In response to environmental stimuli, the bacterium produces and secretes its main virulence factor, the cholera toxin (CT). CT is an AB5 protein toxin, which consists of one toxic A-subunit (CTA) and five identical B-subunits arranged in a doughnut-shaped ring (CTB). The primary receptor of the cholera toxin is the GM1 ganglioside, which is expressed in distinct membrane microdomains of small-intestinal epithelial cells. There are two major biotypes of V. cholerae, classical and El Tor, which produce cholera toxins with a slight sequence variation (cCT and ET CT). cCT and ET CT differ in only two residues of the B-subunit, His18/Tyr18 and Thr47/Ile47 (classical/El Tor).

Crystal structures of the cCTB and ET CTB complexes with A-penta-BGA were determined to a resolution of 1.4 Å and 1.6 Å, respectively. In both structures, A-penta-BGA is bound with the blood-group-A-specific GalNAc residue facing amino acid 18, and with its reducing end (N-acetylglucosamine; GlcNAc) towards residue 47. In the ET CTB structure, only three of the ten binding sites exhibited sufficient electron density to allow modeling of the entire ligand. Even in those cases, the B-factors of the terminal carbohydrate residues GalNAc and Fucα2 were disproportionally high compared to those in the other structures, suggesting that they are less tightly bound (in cCTB, the electron density of the GalNAc residue is slightly better defined). The main differences between the cCTB and ET CTB structures concern the internal Gal residue, which interacts with Tyr18 and His94 in the ET CTB structure, while in cCTB, it is too far away from the shorter His18 side chain to form a hydrogen bond. It is noteworthy that in the ET CTB structure exclusively, Gln16 often has a different conformation and points away from the ligand-binding site, thereby weakening the H-bonding network to the ligand. In the ET CTB crystal structure, only three of ten binding sites showed sufficient electron density to warrant modeling of the entire A-penta-BGA ligand, and even then, the GalNAc residue characteristic of blood group A was disordered. Notably, the GalNAc residue is close to Tyr18 and not Ile47, the substitution of which restored binding activity. In the crystal structure of ET CTB in complex with A-penta-HMO, the GalNAc residue is, however, well defined by electron density, strongly suggesting that interference of the reducing end N-acetyl group with Ile47 is responsible for the weaker binding affinity of A-penta-BGA versus A-penta-HMO and ET CTB versus ET CTB I47T/cCTB/LTB. In addition, we observe a conformational change of Gln16 upon binding of A-penta (BGA or HMO), which suggests that this residue interferes with binding in its native conformation.

>TPQNITDLCAEYHNTQIYTLNDKIFSYTESLAGKREMAIITFKNGAIFQVEVPGSQHIDSQKKAIERMKDTLRIAYLTEAKVEKLCVWNNKTPHAIAAISMAN[10x]>[14x]NPLIAAASVIAAGLAVGLASIGPGVGQGTAAGQAVEGIARQPEAEGKIRGTLLL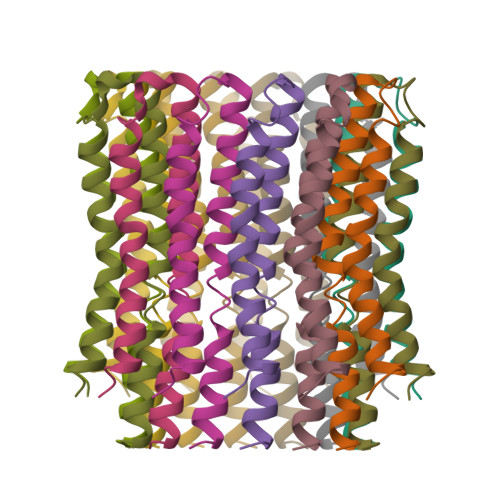SLAFMEALTIYGLVVALALLFANP>[3x]MITTKTVNGVQIAFDDQGHEPGPVFVTLSGWAHDLRAYDGMLPYLRAAQRTVRVCWRGHGPDRNLVGDFGIDEMAADTIGLLDALEVDSFVPIAHAHGGWAALEIADRLGAQRVPAVMILDLIMTPAPREFVAALHGIQDPERWKEGRDGLVQSWLAGTTNQ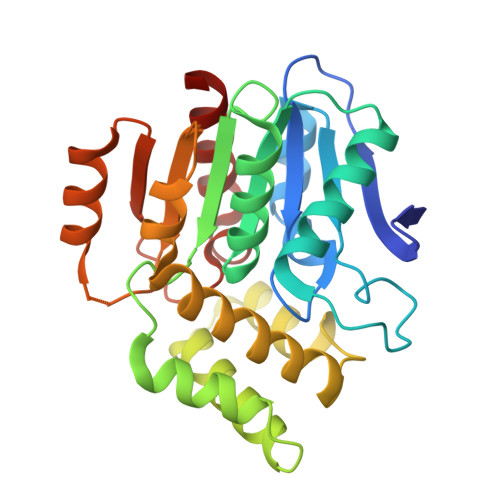AVLDHVRYDSGGHGFDMWARAGRVIDEAYRTWGSPMRRMEALAEPCAIRHVFSHPKIGEYDALHDDFAARHPWFSYRRLGGETHFPGIELPQQVAAEAIDLLAGARI>[2x]AGFQLNEFSSSGLGRAYSGEGAIADDAGNVSRAPALI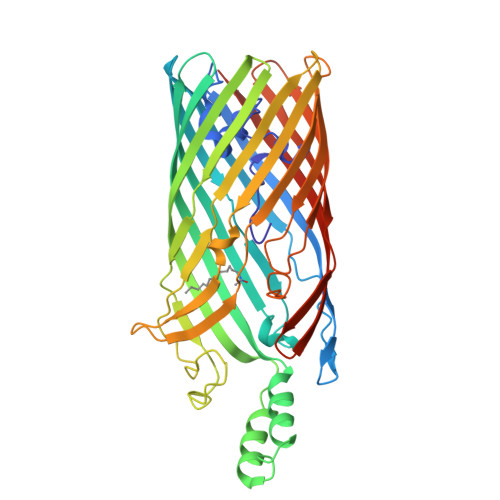TMFDRPTFSAGAVYIDPDVNISGTSPSGRSLKADNIAPTAWVPNMHFVAPINDQFGWGASITSNYGLATEFNDTYAGGSVGGTTDLETMNLNLSGAYRLNNAWSFGLGFNAVYARAKIERFAGDLGQLVAGQIMQSPAGQTQQGQALAATANGIDSNTKTAHLNGNQWGFGWNAGILYELDKNNRYALTYRSEVKIDFKGNYSSDLNRAFNNYGLPIPTATGGATQSGYLTLNLPEMWEVSGYNRVDPQWAIHYSLAYTSWSQFQQLKATSTSGDTLFQKHEGFKDAYRIALGTTYYYDDNWTFRTGIAFDDSPVPAQNRSISIPDQDRFWLSAGTTYAFNKDASVDVGVSYMHGQSVKINEGPYQFESEGKAWLFGTNFNYAFHHHHHH> GPVWRKHYITYRINNY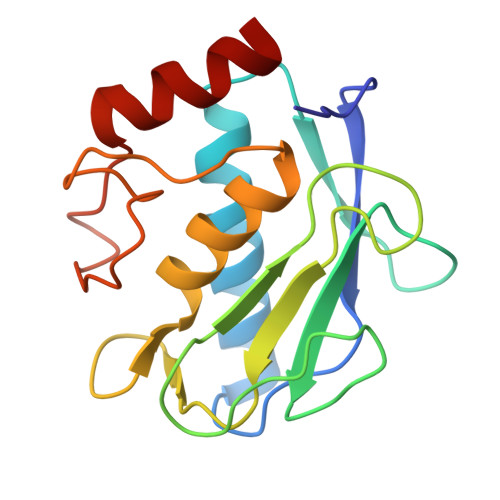TPDMNREDVDYAIRKAFQVWSNVTPLKFSKINTGMADILVVFARGAHGDDHAFDGKGGILAHAFGPGSGIGGDAHFDEDEFWTTHSGGTNLFLTAVHEIGHSLGLGHSSDPKAVMFPTYKYVDINTFRLSADDIRGIQSLYG> NNNFFDPKLMSDWEDEDLDTDNDNIPDSYERNGYTIKDLIAVKWEDSFAEQGYKKYVSNYLESNTAGDPYTDYEKASGSFDKAIKTEARDPLVAAYPIVGVGMEKLIISTNEHASTDQGKTVSRATTNSKTESNTAGVSVNVGYQNGFTANVTTNYSHTTDNSTAVQDSNGESWNTGLSINKGESAYINANVRYYNTGTAPMYKVTPTTNLVLDGDTLSTIKAQENQIGNNLSPGDTYPKKGLSPLALNTMDQFSSRLIPINYDQLKKLDAGKQIKLETTQVSGNFGTKNSSGQIVTEGNSWSDYISQIDSISASIILDTENESYERRVTAKNLQDPEDKTPELTIGEAIEKAFGATKKDGLLYFNDIPIDESCVELIFDDNTANKIKDSLKTLSDKKIYNVKLERGMNILIKTPTYFTNFDDYNNYPSTWSNVNTTNQDGLQGSANKLNGETKIKIPMSELKPYKRYVFSGYSKDPLTSNSIIVKIKAKEEKTDYLVPEQGYTKFSYEFETTEKDSSNIEITLIGSGTTYLDNLSITELNSTPEILDEP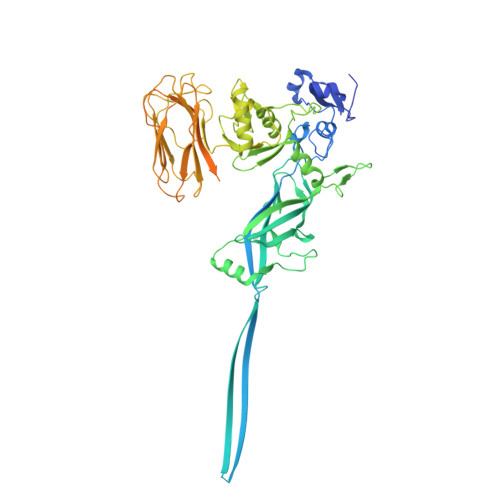EVKIPTDQEIMDAHKIYFADLNFNPSTGNTYINGMYFAPTQTNKEALDYIQKYRVEATLQYSGFKDIGTKDKEMRNYLGDPNQPKTNYVNLRSYFTGGENIMTYKKLRIYAITPDDRELLVLSVD>MKQKVHSVSYLAKAEFKFNNGVYNLVALPSGAEVVKVSLEVVGNPIATSTTSVSVGFEDETTKNYFLTLDNLAVDDASKKHTTSAKDYTATSNKVVVAEVKNANDNNVKGVLRVLYFLPSVIEVEY[9x];>MLEKLNNINFNNISNNLNLGIEVGREIQNASWIKSPFFSITGTGADRGVRLFSVASQQPFRPRIKAQ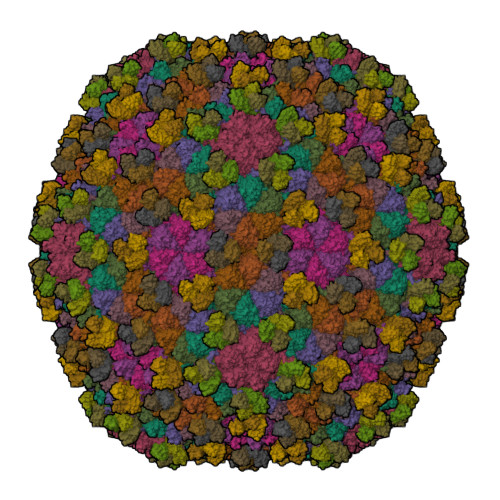LSGSGVSGNTDFEANYDNLEILSQTIYPDAFGNSLRSKIKAYSELERIDFIKESVDSLTTWMNEERDKRIVASLTNDFTNYLYTQTMNVATIRKAIFHARNGLKGDNSKAFPIKPIRATMQSVGNVMVQNTSYIILLDSYQANQLKADSEFKELRKLYAFAGEDKGMLYSGLLGVIDNCPVIDAGVWNKFNVGMPNSSISDSDFMRYLNKANVSSIVTPRQFKEKLNQEKDEKKRSINKEISIGCLIGASAVLLAGSKETRFYIDETVDAGRKSLVGVDCLLGVSKARYQSTDGVVTPYDNQDYAVIGLVSDME[9x]Thioredoxins (TRXs) are small oxidoreductases that contribute, in most living organisms, to the control of cellular redox homeostasis. Indeed, they reduce disulfide bonds on numerous proteins involved in several processes, including antioxidant defense mechanisms, photosynthetic carbon metabolism, and protein folding. In addition, TRXs have been suggested to control two additional Cys-based post-translational modifications, namely S-glutathionylation and S-nitrosylation, by catalyzing the reduction of glutathione-mixed disulfides (–SSGs) and S-nitrosothiols (–SNOs), respectively. The redox activity of TRXs relies on the presence of two Cys residues in the conserved Trp-Cys-(Gly/Pro)-Pro-Cys (WC(G/P)PC) active site motif.

In the present study, we deepen the structural features of CrTRXh1, providing the 3D structures of both the reduced form and variants in which catalytic cysteines were mutated. Regardless of the reducing activity in which TRXs are involved, the N-terminal active site Cys (CysN) is responsible for the first nucleophilic attack on oxidized targets. While the subsequent catalytic steps underlying TRX-dependent protein deglutathionylation and denitrosylation are yet undefined, the reduction of protein disulfides implies the formation of a mixed-disulfide bond between the CysN and a Cys on target protein.

> MGGSVIVIDSKAAWDAQLAKGKEEHKPIVVDFTATWSGPCKMIAPLFETLSNDYAGKVIFLKVDVDAVAAVAEAAGITAMPTFHVYKDGVKADDLVGASQDKLKALVAKHAAA> APQVVDKVAAVVNNGVVLESDVDGLMQSVKLNAAQARQQLPDDATLRHQIMERLIMDQIILQMGQKMGVKISDEQLDQAIANIAKQNNMTLDQMRSRLAYDGLNYNTYRNQIRKEMIISEVRNNEVRRRITILPQEVESLAQQVGNQNDASTELNLSHILIPLPENPTSDQVNEAESQARAIVDQARNGADFGKLAIAHSADQQALNGGQMGWGRIQELPGIFAQALSTAKKGDIVGPIRSGVGFHILKVNDLRGESKNISAAQKDRAYRMLMNRKFSE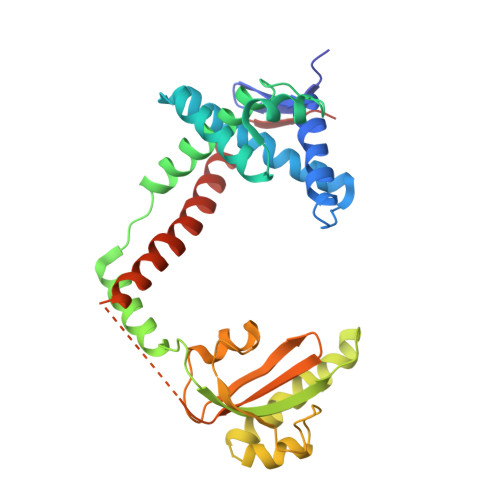EAASWMQEQRASAYVKILSN>SEKPVYLSVKADNSMFIGNDPVTDETMITALNALTEGKKDTTIFFRADKTVDYETLMKVMDTLHQAGYLKIGLVGEETAKAK[2x];> KKAQPISVTMVTPADLEPPQAKK

Active nutrient uptake is fundamental for survival and pathogenicity of Gram-negative bacteria, which operate a multi-protein Ton system to transport essential nutrients like metals and vitamins. One of the key systems involved in this transport is the Ton system, which forms a multi-protein complex embedded in the inner membrane. This system utilizes the proton motive force (PMF) to physically open a variety of outer membrane transporters – the so-called TonB-dependent transporters (TBDTs) – and, hereby, realizes active transport by means of the inner membrane proton channel-forming complex ExbB-ExbD and the periplasm crossing protein TonB. Here, we study the periplasmic domain of ExbD, a crucial component of the proton channel of the Ton system. We show that this domain is a dynamic dimer switching between two conformations representing the proton channel’s open and closed states.

Herein, we initially hypothesized that TonB/HasB might bind between the two protomers of ExbD, effectively replacing the NIBS residues at the dimer interface. This idea was driven by our observation that the NIBS residues unfold upon addition of TonB/HasB, implying a potential competition between the NIBS residues and HasB/TonB for the same binding site. To investigate this possibility, we solved the crystal structure of an ExbD construct lacking the N-terminal residues 43-60 (ExbDEc, ΔNIBS) in complex with the corresponding TonB peptide at 1.5 Å resolution. The crystal structure confirms that the IDR of TonB undergoes a disorder-to-order transition upon binding to ExbD, replacing the NIBS residues in between the two ExbD protomers. In this arrangement, the TonB peptide forms an intermolecular β-sheet: A parallel β-sheet with the β6-strand of one protomer, and an antiparallel β-sheet with the β6-strand of the second one. Corroborating these structural observations, AUC experiments of ExbDEc, peri and the TonB peptide confirm that ExbD retains its dimeric structure in solution upon binding to the IDR. Upon encountering HasB/TonB, this open state is conformationally selected through the binding of HasB/TonB into the groove between the two protomers, which was previously occupied by the now-unfolded NIBS. This would mark a critical first step in the activation of the system. The open state of ExbD is selectively bound by an IDR of the partner proteins TonB/HasB, which undergo a disorder-to-order transition as they bind between the two ExbD protomers, as evidenced by X-ray crystallography. However, we showed that the transition between the open and closed states of ExbD operates at distinct rates in these systems: on the slow NMR time scale (ms) for the single-target Has system and in the intermediate time scale (μs-ms) for the multi-target Ton system.>[10x]MFLKAVVLTLALVAVAGARAEVSADQVATVMWDYFSQLSNNAKEAVEHLQKSELTQQLNALFQDKLGEVNTYAGDLQKKLVPFATELHERLAKDSEKLKEEIGKELEELRARLLPHANEVSQKIGDNLRELQQRLEPYADQLRTQVSTQAEQLRRQLTPYAQRMERVLRENADSLQASLRPHADELKAKIDQNVEELKGRLTPYADEFKVKID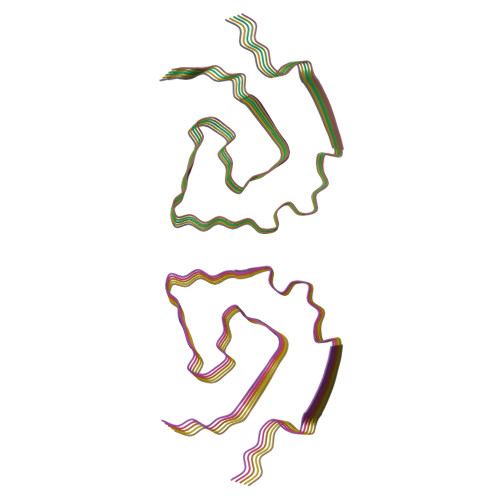QTVEELRRSLAPYAQDTQEKLNHQLEGLTFQMKKNAEELKARISASAEELRQRLAPLAEDVRGNLRGNTEGLQKSLAELGGHLDQQVEEFRRRVEPYGENFNKALVQQMEQLRQKLGPHAGDVEGHLSFLEKDLRDKVNSFFSTFKEKESQDKTLSLPELEQQQEQQQEQQQEQVQMLAPLES The degradation of HIFα subunits is promoted by post-translational hydroxylation of prolyl-residues located in its N/C-terminal oxygen dependent degradation domains (NODD and CODD). These dioxygen-sensitive reactions are catalysed by 2-oxoglutarate (2OG) and Fe(II) dependent prolyl hydroxylases (PHD 1–3 in humans). The human PHDs catalyse hydroxylation of prolyl-residues within the N/C terminal ODDs of HIF-1/2/3α and are negative regulators of the transcriptionally regulated hypoxic response.

Following from the observation that specific heteroaromatic inhibitors with glycine side chains induce PHD2 crystallization in the P63 form, we investigated the selectivity of small-molecule induced PHD2 crystallization. We employed 96-well screens for crystallizing PHD2 constructs (PHD2181-426 and PHD2181-407, hereafter nPHD2 and cPHD2, respectively) with a set of cyclic 2OG analogues and related small-molecules. We observed that crystallization of nPHD2 is induced by succinamic acid derivatives (SCAs), 4a, 4b, 7f. and 30a. This is interesting because none of these SCAs are potent PHD2 inhibitors or stabilizers (as observed by MS, NMR and thermal shift analyses) in solution. The nPHD2.SCA complex structures manifest a similar ligand binding mode to that observed in the reported nPHD2.FG2216/P63 structures, i.e. like FG2216 and related compounds, the SCAs coordinate the active site metal ion via their heteroaromatic ring nitrogen and side chain amide carbonyl oxygen. However, while the bidentate coordination of the active site metal ion by SCAs forms an approximately planar six-membered chelate ring, more established PHD inhibitors, including FG2216, form a five-membered chelate ring. The chelate ring size may affect the stability of the protein-complex and possibly its binding/inhibition potential. Although biophysical (MS, NMR) analyses suggest that SCAs form only a weak complex with monomeric nPHD2, the clear Fo-Fc difference density for the SCAs suggests that intermolecular interactions of SCAs notably with the C-terminus of a threefold symmetry related neighbour in the P63 form may both stabilize the ligand binding in the crystal lattice and help promote crystallization. Unexpectedly, the work with small molecule ligands led to the observation that the ability to induce formation of the homotrimeic crystal form does not correlate with either their active site ligand binding efficiency or inhibitory potency. Compounds from both the FG2216 and SCA series enable nPHD2 crystallization with approximately equal efficiency, yet FG2216 (and related compounds) are significantly more potent inhibitors than the SCAs under the tested assay conditions.

> GSHMASPNGQTKPLPALKLALEYIVPCMNKHGICVVDDFLGKETGQQIGDEVRALHDTGKFTDGQLVSQKSDSSKDIRGDKITWIEGKEPGCETIGLLMSSMDDLIRHCNGKLGSYKINGRTKAMVACYPGNGTGYVRHVDNPNGDGRCVTCIYYLNKDWDAKVSGGILRIFPEGKAQFADIEPKFDRLLFFWSDRRNPHEVQPAYATRYAITVWYFDADERARAKVKYLTGEKGVRVELNKPSDSVGKDVF> MYKKIIAVAALFCASIGILKGQSSDLTPQDTIYSPEISYAKPIHKTIASIEIEGMRSFDDFVLRNLSGLAVGDEVLIPGDAMSAAVNRIMRQGYFSNVRIIADKYVGNKVYLKIIVTERPRISKVTFSGVKKSEREDLEMKIGLREGIQMTRNNEDKVRQIVQKYFSEKGYRDASIRITQEPDLSKDGFVNVLISIEKKSKTKVNEIYFSGNKALSNHKLRMAMKNTNAKFSLRKHIRSSFLKLFSTHKFVEESYREDLVRLIEKYQEYGYRDAEILTDSVVKAPDGKRVDIYLNIEEGQKYYIKDVNFVGNSQYPSEYLERVLGIKSGDVYNQRRLAKRLNEDEDAVGNLYYNNGYIFAWVDPVETNVVGDSVSLDIRIAEGKQANINKVIIKGNTVVYEDVVRRELYTKPGQLFSREDIINSIRLINQLGHFDAEKSIPRPIPNPETGTVDIEYDLVPRSSDQLELSVGWSQSGLLFRGAIKFTNFSVGNLLHPSMYKKGIIPQGDGQTLSLSAQTNGKYYQQYSVTFMDPWFGGKRPDMFSFSAFYSKTTAIDSKFYNSNAGNYYNAYYNSYYNNYNSYYNGMSNYTGDLYTQASDPDRSLQMLGTSIGYGKRLTWPDNWFQIYTSLNYTYYRLRNWSYNTFQNFHHGSANDLNLELRLSRTSIDNPIYTRSGSDFMVSVAATLPYSLWDNHDYASQNLSVSDRYRYIEYHKWKFRGRVFTPLLNPATHKYTPVLMSRVEGAVLGSYNSNKKSPFGTFYMGGDGMSSYYGGYMNETIGLRGYKNGSIAGNNYDYAYAYMRLTMELRFPILFENSFNAWLLAFAEAGNAWRSIDNYNPFNLKRSAGVGLRVTLPMVGMLGIDWGYGFDRPDNSLQRGGSNVHFVLGQEF;> MYKDYKGLYASLRWCALIIGLLFAADSIQAQNNNFTESPYTRFGLGRLGERTTISGHSMGGLGVGLRQGTYVNAVNPASYSAVDSMTFIFDFGASTGITWYAENGKKDNRKMGNIEYFAMLFPISKSIAMSAGVLPYSASGYQFGSVDQVEGGSVQYTRKYLGTGNLNDLYVGIGATPFKNFSIGANASFLFGRFTHSRQVIFSTEAPYNPVHLSTLYLKAAKFDFGMQYHLPLKSDRSLVIGAVYSPRVKMHSELTQIKNQVQNGVVVESETQEYIKGMDYYTLPHTLGIGFSYEKKDKLLLGADVQYSKWKGEKFYKSDCKFQDRIRVSLGGEIMPDINAVGIWPKVRYRFGLHGENSYLKVPTKGGVYQGYHIVGAVFGIGIPLNDRRSFVNVSLEYDRLIPKEGMIKENALKLTFGLTFNESWFKKLKLN;> MKRYLLLVFSLMALLTVACDDDLSPIGGSIQPPSDPVSARVDTLEFSVKTIPMGDIYNRTNYTLLGDLTDPEYGDLKADYIMQFKSPRNFKFKYPPKDGKIDSVKLSINYDSWAGDSTSIMKVSIYKINKAIPPSYYSTQELASLLDETQIIASQTFKAGNDSAFHRVRIPLPNEIGQKIYDLSVNNPSVFDTQESFYNNVLGGLYVTTTTGTGVVLSVYNTQMAIFYSYKVAADSTATASETFVNTSESYQVNHIKNSQISHLLQENDSLSCVKSPAGVMTQLTISKEQFTDAFTSNLSSSLAWQIGEAQFNISASKPSEGLMLSPPSYLLLLPQDSVRNFFEQEQTELMQPRTAFLSTIYNIKKREYRFSNISRLLMEHIKNNTEKTPEGKPYITKDLVLVLLPVKRQVAGASNSLYTSQLNNFMFPSGVKLQLGKKNKTARIGVYSMTYTDNHHHHHHH;> MCKKHFIRYFFWTIIVFFVGAAIHSCKESKIDLEEVSIVDLQIHRFYLSSKKNPDLEKVFFSIDHAKGTIINKKYMPYGTVLDSVMMKLVTDFSAKKLRVAINDGEYKDWHNKDSLWLRDCHTLHLMVFDESGEKTKKYTVTLNRYDYQPTTFVWHMLDGVALPDINASFVDVVTHADKVYLVAATGNKTLLYSSDRKNPVHWTLLSSSGLSGACRQIAATEDGRAWILTDSGIYQSDDFTNWSLLPSEVPVTTLLGAMAWPQGSHTLALLAEKEGSLFFATNIDGIHSWQEQAPETFPVRNFSTQLYKANNHPMLRLVGGVTHTGAPATSVWITSNGNDWFGLDLAAGAIPASMEKGALVQTPSDGNLYYYATEQAEGIKRVAVAYSTDKGITWKRGAADIMLPADPFYTVGYPLPFVCAFDDGAYNIYQLGGVSSSGTFFSSIWKGILKLNENN;> MKTKKNIIMALGLMLVNILLVFSSCEKRPNEEKQRRHDNEVAFNAYADSTNFKKVSVDGSTAYVYMRWITNGTGTEHPIATSRVEVHYQTYRLVGNIMVDGNYNSEKPARITLYRNEKDKSITGFRIALQNMVIGDECEFIVPWYLAYGSKGVPASSANLVPIPSYSALRFIVKLSGIIPEEDKK;> MKRIIMILLPVLAIGMAVLTLGSCKKSDIKSLKEMKKDERKAIESFINRMGFTIKEGHEGQSEFDPDIMYHFDNDLYMQVLDKGKEPPVLNKTKINVRMEGFMFNRERDSIYVFNSLTSGGFQESVFRYIYKYNDGDIHFELIKCTTGSNLDMFVCEGVAFPMTMLGNKARVRLIVPFRIGPESLYSRGLTGYYKEVEYVFRD

The β-barrel assembly machinery (BAM) complex is a conserved, multiprotein machine that mediates the folding and membrane insertion of newly synthesized β-barrel outer membrane (OM) proteins. Cryogenic electron microscopy (cryo-EM) structures of the BAM complexes from the gut commensal B. thetaiotaomicron and the oral pathogen Porphyromonas gingivalis are similar and reveal a 7-protein, ~325-kDa complex with most of its mass on the extracellular side. Remarkably, besides BamA and BamD subunits, Bacteroidetal BAM contains a 14-stranded integral OMP that is intimately associated with BamA. The remaining four components, named BamH–K, are all SLPs and form an extracellular dome-like structure over BamA that may provide additional functionality to enable the folding and assembly of the many β-barrel–SLP complexes that are a hallmark of the Bacteroidota.

Tagging PgBamA at the N-terminus led to low yields of intact complex owing to proteolytic degradation of the periplasmic domain, presumably by the ubiquitous gingipain surface proteases characteristic of P. gingivalis. A tag added to the C-terminus of PgBamH (PGN_1735) allowed us to purify the intact complex and determine its cryo-EM structure at ~3.2 Å resolution. The composition and architecture of the PgBAM complex is very similar to that of B. thetaiotaomicron, with a pronounced extracellular dome formed by BamG–K. Only very weak, not modelled, density was observed for the periplasmic components, possibly owing to clipping by gingipains, similar to what was observed in the isolation of tagged PgBamA. All components of PgBAM and BtBAM are similar in size except for BamH, which is 88 residues longer in B. thetaiotaomicron. Structural alignments of individual BtBAM and PgBAM components show high structural similarity for BamAGHIJ. The highest Cα-Cα root mean square deviation (RMSD) of 6.3 Å was observed for BamI, although both PgBamI and BtBamI consist of an N-terminal Ig-like domain and a C-terminal six-bladed β-propeller. The extracellular dome of PgBAM is much more compact than that of BtBAM, as indicated by the distance between the BamJ and BamK PPIs. A total of 12 glycosylation sites are present within PgBAM, mostly located on BamH (7 sites). The tri-acylated PgBamH lipid anchor is clearly defined and, like in B. thetaiotaomicron, positioned at the BamAG interface. EL3 in P. gingivalis BamA is 39 residues long and contains 12 tyrosines.> MTTVSCPANVITTTESDRIAGLFNIPAGIIPTGNVLSTIEVCAHRCIFDFFKQIRSDDNSLYSAQFDILLGTYCNTLNFVRFLELGLSVACICTKFPELAYVRDGVIQFEVQQPMIARDGPHPVDQPVHNYMVKRIHKRSLSAAFAIASEALSLLSNTYVDGTEIDSSLRIRAIQQMARNLRTVLDSFERGTADQLLGVLLEKAPPLSLLSPINKFQPEGHLNRVARAALLSDLKRRVCADMFFMTRHAREPRLISAYLSDMVSCTQPSVMVSRITHTNTRGRQVDGVLVTTATLKRQLLQGILQIDDTAADVPVTYGEMVLQGTNLVTALVMGKAVRGMDDVARHLLDITDPNTLNIPSIPPQSNSDSTTAGLPVNARVPADLVIVGDKLVFLEALERRVYQATRVAYPLIGNIDITFIMPMGVFQANSMDRYTRHAGDFSTVSEQDPRQFPPQGIFFYNKDGILTQLTLRDAMGTICHSSLLDVEATLVALRQQHLDRQCYFGVYVAEGTEDTLDVQMGRFMETWADMMPHHPHWVNEHLTILQFIAPSNPRLRFELNPAFDFFVAPGDVDLPGPQRPPEAMPTVNATLRIINGNIPVPLCPISFRDCRGTQLGLGRHTMTPATIKAVKDTFEDRAYPTIFYMLEAVIHGNERNFCALLRLLTQCIRGYWEQSHRVAFVNNFHMLMYITTYLGNGELPEVCINIYRDLLQHVRALRQTITDFT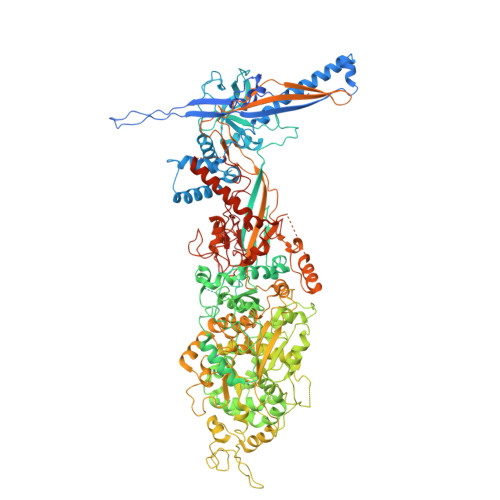IQGEGHNGETSEALNNILTDDTFIAPILWDCDALIYRDEAARDRLPAIRVSGRNGYQALHFVDMAGHNFQRRDNVLIHGRPVRGDTGQGIPITPHHDREWGILSKIYYYIVIPAFSRGSCCTMGVRYDRLYPALQAVIVPEIPADEEAPTTPEDPRHPLHAHQLVPNSLNVYFHNAHLTVDGDALLTLQELMGDMAERTTAILVSSAPDAGAATATTRNMRIYDGALYHGLIMMAYQAYDETIATGTFFYPVPVNPLFACPEHLASLRGMTNARRVLAKMVPPIPPFLGANHHATIRQPVAYHVTHSKSDFNTLTYSLLGGYFKFTPISLTHQLRTGFHPGIAFTVVRQDRFATEQLLYAERASESYFVGQIQVHHHDAIGGVNFTLTQPRAHVDLGVGYTAVCATAALRCPLTDMGNTAQNLFFSRGGVPMLHDNVTESLRRITASGGRLNPTEPLPIFGGLRPATSAGIARGQASVCEFVAMPVSTDLQYFRTACNPRGRASGMLYMGDRDADIEAIMFDHTQSDVAYTDRATLNPWASQKHSYGDRLYNGTYNLTGASPIYSPCFKFFTPAEVNTNCNTLDRLLMEAKAVASQSSTDTEYQFKRPPGSTEMTQDPCGLFQEAYPPLCSSDAAMLRTAHAGETGADEVHLAQYLIRDASPLRGCLPLPR> ADLGSKNLKSPQKVEVDIIDDNFILRWNRSDESVGNVTFSFDYQKTGMDNWIKLSGCQNITSTKCNFSSLKLNVYEEIKLRIRAEKENTSSWYEVDSFTPFRKAQIGPPEVHLEAEDKAIVIHISPGTKDSVMWALDGLSFTYSLVIWKNSSGVEERIENIYSRHKIYKLSPETTYCLKVKAALLTSWKIGVYSPVHCIKTTVENELPPPENIEVSVQNQNYVLKWDYTYANMTFQVQWLHAFLKRNPGNHLYKWKQIPDCENVKTTQCVFPQNVFQKGIYLLRVQASDGNNTSFWSEEIKFDTEIQAFLLPPVFNIRSLSDSFHIYIGAPK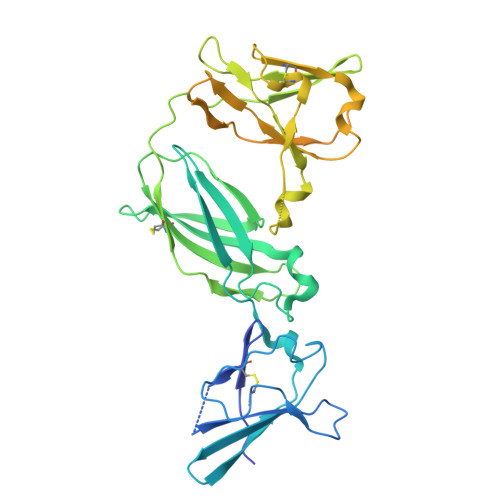QSGNTPVIQDYPLIYEIIFWENTSNAERKIIEKKTDVTVPNLKPLTVYCVKARAHTMDEKLNKSSVFSDAVCEKTKPGNTSK>[2x]MMALRTLSALPVFADSLFSDRFNRIDR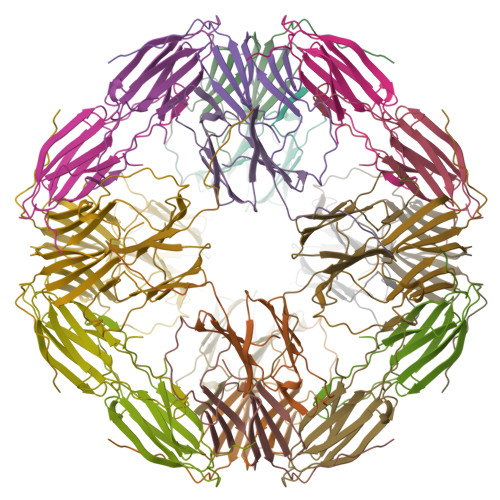LFSQLTGDTPVAATPAYDLQKRDANNYLLTVSVPGWKEEELEIETVGGNLNITGKHTEETVEDQTHWIYRGIRKADFQLSFSLPEHAKVNNAKLEQGLLLVEIYQEIPESEKPKKIAIES>MAHHHHHHSSGLEVLFQGPMTHSVVELIEIESAIIQVKMQDRTHKNAFSQELTDDLIQAFEYIRQNPKYKAVILTGYDNYFASGGTQEGLLRIQQGLTKFTDDNLYSLALDCEIPVIAAMQGHGIGGGFVMGLFADIVILSRESVYTANFMKYGFTPGMGATFIVPKKLGFSLAQEILLNAGSYRGADLEKRGVPFKVLPRAEVLDYAVELAQELAEKPRNSLVTLKDHLVAPLRDQLPRVIEQELMMAEKTFHHEEVKSRIKGLYGN[3x]

In this study we present a structural and functional description of the bacillaene synthase β-branching enzymes PksH and PksI. These biocatalysts are responsible for the final two steps in β-methyl branch incorporation in this PKS/NRPS pathway. There is a single active site per PksI monomer, with each active site positioned on the periphery of the trimer, ~ 43 Å from one other. Akin to PksH, PksI adopts a characteristic CS fold, with a ββα core, that comprises two approximately perpendicular -sheets surrounded by -helices.

Assays were conducted using WT PksI, along with the point mutants PksI-H230A, PksI-H235A, PksI-K80A, PksI-K232A. Of the four PksI mutants investigated only PksI-H230A was found to be catalytically compromised, with barely detectable activity for 3-methyl glutaconyl-SNAC and significantly impaired activity for 3-methyl glutaconyl-CoA. Surprisingly, PksI-K80A and PksI-K232A both display catalytic activities akin to that of WT-PksI, with no evidence of functional impairment. In tandem with kinetic assays, the crystal structures of PksI-K80A, PksI-K232A and H230A were determined. The active sites of each of these enzymes displays the ground state “closed” conformation as observed in the WT enzyme, with no evidence of significant structural perturbations within the active site. These data thus imply that the observed kinetic effects are not attributable to global or local structural reorganization within the enzyme as a consequence of the amino acid substitutions made. Crystal structures of the mutants PksI_K80A, PksI K232A and PksI H230A revealed no significant changes in active site architecture beyond side chain identity. We thus propose a His230 dependent mechanism wherein this residue has a dual function both catalyzing decarboxylation and to act as a proton donor to the decarboxylated intermediate 7 to give the reaction product.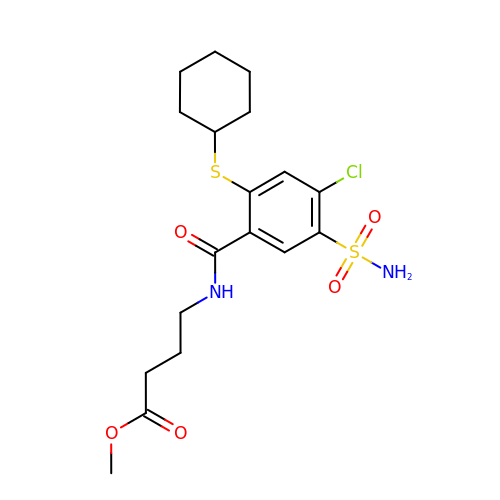methyl 4-[(4-chloranyl-2-cyclohexylsulfanyl-5-sulfamoyl-phenyl)carbonylamino]butanoate | C18 H25 Cl N2 O5 S2 | AUBRGAXHAIBSRT-UHFFFAOYSA-N>[4x]LHRNSLIVLADVALFLALYHFLPFEHNVVLGISMLAFIAVLWLTEALHVTVTAILVPVMAVFFGIFETQAALNNFANSIIFLFLGGFALAAAM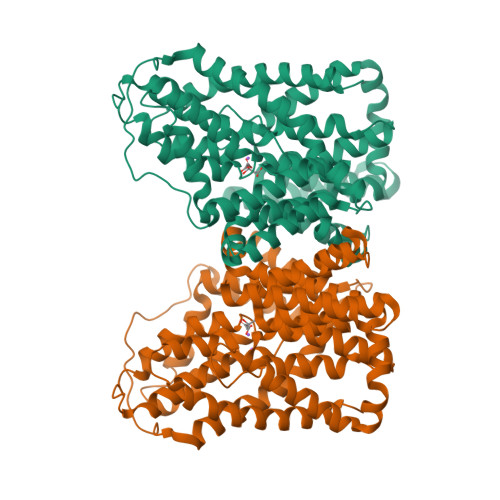HHQGLDKVIADKVLAMAQGKMSVAVFMLFGVTALLSMWISNTATAAMMLPLVLGVLSKVDADKQRSTYVFVLLGVAYSASIGGIATLVGTGPNAIAAAEVGLSFTDWMKFGLPTAMMMLPMAIAILYFLLKPTLNGMFELDRAPVNWDKGKVVTLGIFGLTVFLWIFSSPINAALGGFKSFDTLVALGAILMLSFARVVHWKEIQKTADWGILLLFGGGLCLSNVLKQTGTSVFLANALSDMVSHMGIFVVILVVATFVVFLTEFTSNVATTTLLIPVFATVAEAFGMSPVLLSVLIAVAASCAFMLPVATPPNAIVFASGHIKQSEMMRVGLYLNIACIGLLTAIAMLFWQ>[8x]AGGKVTSSTGIAPKRYVYYPGSEELGPDEIRVIACGTGMPTARRAQAAAAWVVELGNGDKFIVDIGSGSMANIQSLMIPANYLTKIFLTHLATDHWGDLVSMWAGGWTAGRTDPLEVWGPSGSREDMGTKYAVEHMLKAYNWDYMTRAVTINPRPGDINVHEFDYRALNEVVYQE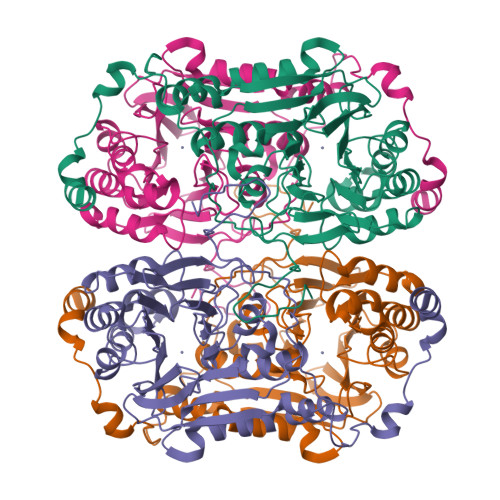NGVTFRSWPCIHAGDGPVSFALEWNGYKVVFGGDTAPNIWYPEYAKGADLAIHECWMTSDQMMTKYNQPAQLALRINLDFHTSAQSFGQIMNMVQPRHAVAYHFFNDDDTRYDIYTGVRENYAGPLSMATDMMVWNITRDAVTERMAVSPDHAWDVAGPSEDLAPDRNRASEYTQYILDGRLNVDEANAHWKQEFMG>[4x]AEEFPVPNGFESAYREVDGVKLHYVKGGQGPLVMLVHGFGQTWYE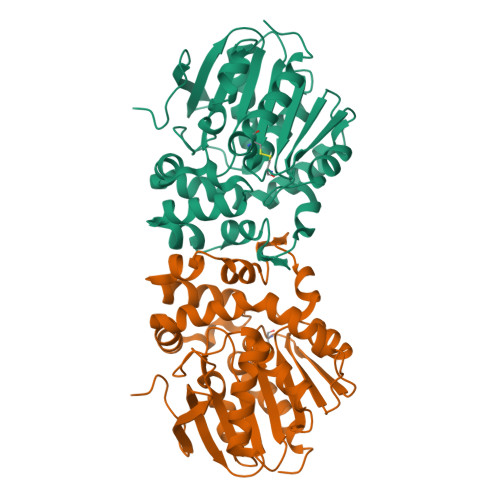WHQLMPELAKRFTVIAPDLPGLGQSEPPKTGYSGEQVAVYLHKLARQFSPDRPFDLVAHDIGIWNTYPMVVKNQADIARLVYMEAPIPDARIYRFPAFTAQGESLVWYFSFFAADDRLAETLIAGKERFFLEHFIKSHASNTEVFSERLLDLYARSYAKPHSLNASFEYYRALNESVRQNAELAKTRLQMPTMTLAGGGHGGMGTFQLEQMKAYAEDVEGHVLPGCGHWLPEECAAPMNRLVIDFLSRGRHHHHHH>[2x]MTKHYDYIAIGGGSGGIASINRAAMYGQKCALIEAKELGGTCVNVGCVPKKVMWHAAQIREAIHMYGPDYGFDTTINKFNWETLIASRTAYID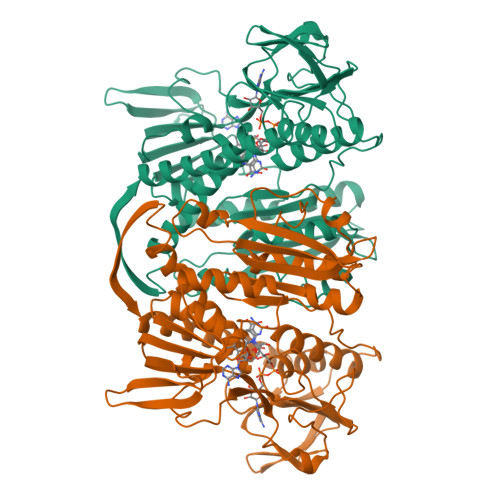RIHTSYENVLGKNNVDVIKGFARFVDAKTLEVNGETITADHILIATGGRPSHPDIPGVEYGIDSDGFFALPALPERVAVVGAGYIGVELGGVINGLGAKTHLFEMFDAPLPSFDPMISETLVEVMNAEGPQLHTNAIPKAVVKNTDGSLTLELEDGRSETVDCLIWAIGREPANDNINLEAAGVKTNEKGYIVVDKYQNTNIEGIYAVGDNTGAVELTPVAVAAGRRLSERLFNNKPDEHLDYSNIPTVVFSHPPIGTVGLTEPQAREQYGDDQVKVYKSSFTAMYTAVTTHRQPCRMKLVCVGSEEKIVGIHGIGFGMDEMLQGFAVALKMGATKKDFDNTVAIHPTAAEEFVTMR>ADPASEEVMACLRQERSRVENPSQTIVNVVAENPAYLHCSVPPDAEHEIAWTRVSDGALLTAGNRTFTRDPRWQVSKKSANIWVLNLRRAEQQDSGCYLCEINDKHNTVYAVYLKVLEPHHHHHH[2x];>[2x]GSGAPPTIQQPSMSSAVALLGQDVDFTCIVNDLGSHMVAFVKADSPPRLLSFDEKVFRRRNKYELKPRIGDLHN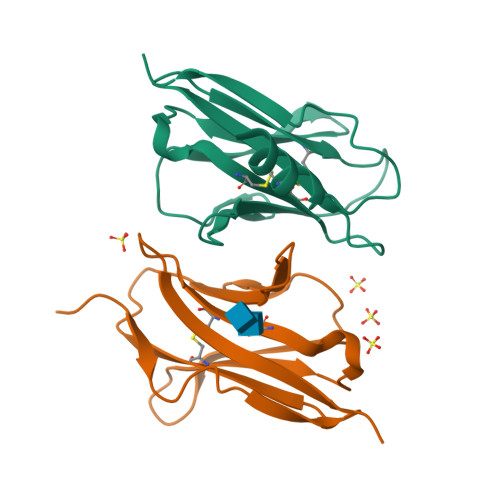EWVLTIKNVQESDRGNYSCQINTEPITLSTGELDVKVPHHHHHH>[2x]MLYIDEFKEAIDKGYILGDTVAIVRKNGKIFDYVLPHEKVRDDEVVTVERVEEVMVELDKLEHHHHHH

Work describing the contribution of bacteriophages to the emergence and diversification of the M1T1 GAS clone revealed that each prophage contains a conserved open reading frame (ORF) of ~60aa named paratox (prx). prx is always located adjacent to a toxin within the prophage, and GAS prophages that lack a toxin also lack prx. In our efforts to study the regulation of natural competence in Streptococcus spp. by ComRS based quorum sensing, we discovered that prx genes contain a perfect CIN-box within their promoter region for recognition by the SigX core-RNA-polymerase complex, and that transcription of prx is induced by XIP. Additionally, we found that Prx binds ComR directly and inhibits activation by XIP both in vitro and in vivo. Taken together we conclude that the conserved prophage protein paratox acts as an inhibitor of new DNA acquisition by pyogenic, bovis and suis streptococci.

Additionally, an X-ray crystal structure of Prx reveals a novel protein fold with only distant structural homologues, which suggests a unique molecular mechanism of ComR-XIP inhibition. Prx crystallized as a dimer in the asymmetric unit. The dimer interface consists of residues from β-strands β1, β3 and the loop region between β2 and β3, which allows the N and C terminal α-helices to be positioned on the same face of the complex. As calculated by MOLEonline/2.531, the pore or cavity sizes are 380Å3 and 993Å3. Although analysis by SEC indicates a possible dimer, analysis with PISA32 gives a complex significance score of 0.1, which suggests a high probability that dimerization is a crystal packing artifact. As demonstrated by analytical ultracentrifugation (AUC), Prx is a monomer (8.39 kDa) in the buffer conditions used in our biochemical experiments. A surface composed of one face of α1 (D5, L8, and E9) and α2 (M55, V46) also cluster into a conserved patch, and both surfaces tend toward an electronegative electrostatic potential. The observed Prx dimer appears superficially similar to a Bateman fold, with each Prx monomer as the individual CBS (cystathionine β-synthase) domain37 as shown in an alignment with human AMP-activated kinase.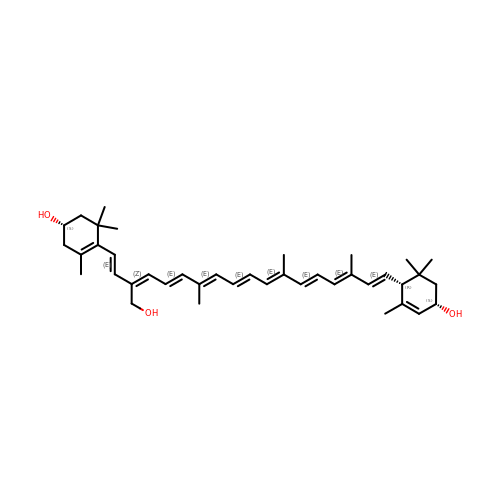(1S)-4-[(1E,3Z,5E,7E,9E,11E,13E,15E,17E)-3-(hydroxymethyl)-7,12,16-trimethyl-18-[(1R,4S)-2,6,6-trimethyl-4-oxidanyl-cyclohex-2-en-1-yl]octadeca-1,3,5,7,9,11,13,15,17-nonaenyl]-3,5,5-trimethyl-cyclohex-3-en-1-ol | C40 H56 O3 | ODGGKCNQKSEQNL-VVAGNOCPSA-N>MEPNPTTIAFQVDCYLWHLKKTLSMMGEVDAPFEDRLRREQKALKGRSMTLGI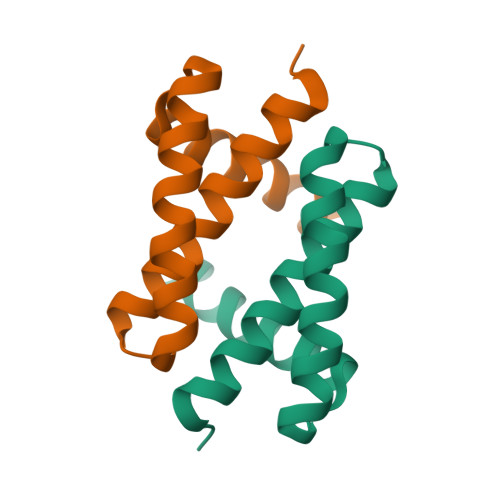DIQSATQEGYYKIKSITEESM[2x]>[12x]MYQLFEELGKGAFSVVRRCVKVLAGQEYAAKIINTKKLSARDHQKLEREARICRLLKHPNIVRLHDSISEEGHHYLIFDLVTGGELFEDIVAREYYSEADASHCIQQILEAVLHCHQMGVVHRDLKPENLLLASKLKGAAVKLADFGLAIEVEGEQQAWFGFAGTPGYLSPEVLRKDPYGKPVDLWACGVILYILLVGYPPFWDEDQHRLYQQIKAGAYDFPSPEWDTVTPEAKDL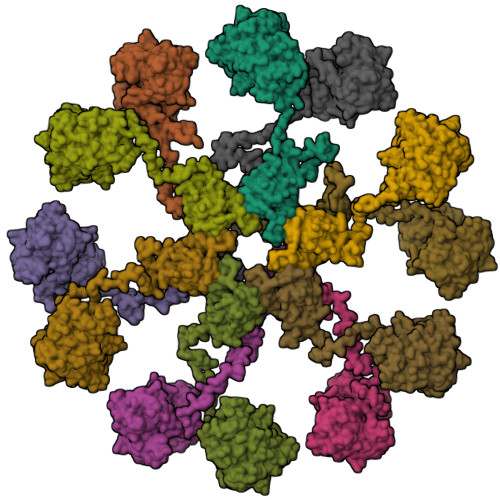INKMLTINPSKRITAAEALKHPWISHRSTVASCMHRQETVDCLKKFNARRKLKGAILTTMLATRNFSGGKSGGNKKSDGVKESSESTNTTIEDEDTKVRKQEIIKVTEQLIEAISNGDFESYTKMCDPGMTAFEPEALGNLVEGLDFHRFYFENLWSRNSKPVHTTILNPHIHLMGDESACIAYIRITQYLDAGGIPRTAQSEETRVWHRRDGKWQIVHFHRSGA>GHMKHTIDPSSPDFQPIPSFEECFPKSTKEHKEVVHEESGHVLKVPFRRVHLSGGEPAFDNYDTSGPQNVNAHIGLAKLRKEWIDRREKLGTPRYTQMYYAKQGIITEEMLYCATREKLDPEFVRSEVARGRAIIPSNKKHLELEPMIVGRKFLVKVNANIGNSAVASSIEEEVYKVQWATMWGADTIMDLSTGRHIHETREWILRNSAVPVGTVPIYQALEKVDGIAENLNWEVFRETLIEQAEQGVDYFTIHAGVLLRYIPLTAKRLTGIVSRGGSIHAKWCLAYHKENFAYEHWDDILDICNQYDVALSIGDGLRPGSIYDANDTAQFAELLTQGELTRRAWEKDVQVMNEGPGHVPMHKIPENMQKQLEWCNEAPFYTLGPLTTDIAPGYDHITSAIGAANIGALGTALLCYVTPKEHLGLPNRDDVKAGVIAYKIAAHAADLAKQHPHAQAWDDAL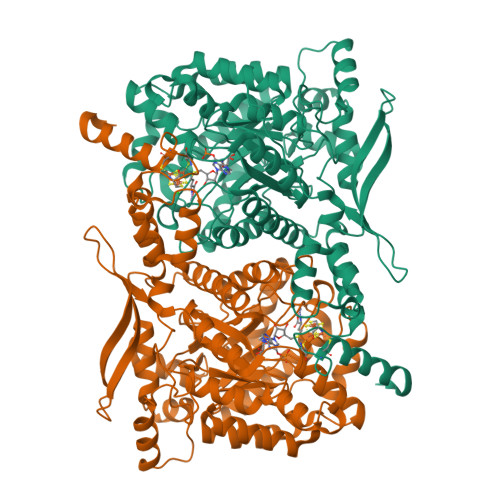SKARFEFRWMDQFALSLDPMTAMSFHDETLPADGAKVAHFCSMCGPKFCSMKITEDIRKYAEENGYGSAEEAIRQGMDAMSEEFNIAKKTISGEQHGEVGGEIYLPESYVKAAQK[2x]>MRSRRVDVMDVMNRLILAMDLMNRDDALRVTGEVREYIDTVKIGYPLVLSEGMDIIAEFRKRFGCRIIADFKVADIPETNEKICRATFKAGADAIIVHGFPGADSVRACLNVAEEMGREVFLLTEMSHPGAEMFIQGAADEIARMGVDLGVKNYSGPSTRPERLSRLREIIGQDSFLISPGVGAQGGDPG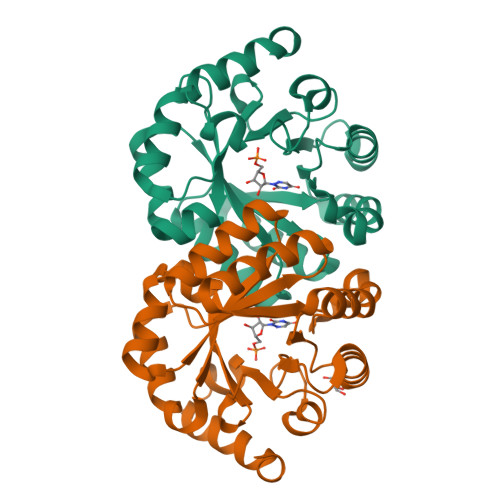ETLRFADAIIVGRSIYLADNPAAAAAGIIESIKDLLNP[2x]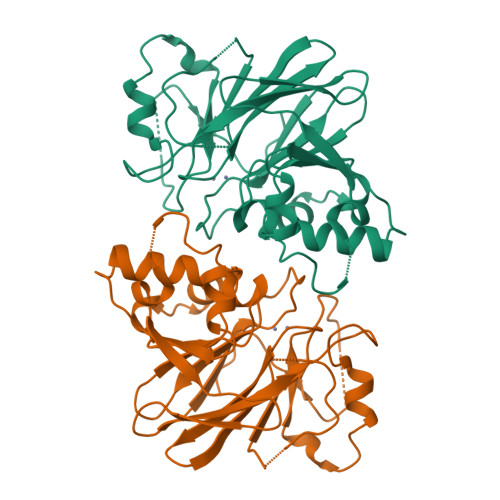> SMLHTTQIRMVGTGSAFSKKFYNNSALVTFTNGYNLLIDCGHSVPKGLHDADIPLESIDGILITHTHADHIGGLEEVALYNKFVLGGRKIDLLVPNTLVESLWENSLKGGLRYSDTYDDLSLSDYFTVRSLKTFTSGAARTQLEENIAIKLYPTFHVSHMASYAVGLEDRGEDKVFYSSDTIFDEYLIDYALTYSWVFHDCQFFTGGVHASLDELLNYIPEEDQDRVFLMHYGDNMEDFFTKTGRMRFALQGRTYIL> MGLNFFRKAAPEVRTEPVAERKASVTGRIVAMASGAGRPVWGPRDTVSLMRTGFAGNPVGFRSVKLIAEATAAVPLICQDAERRYEIHPVLDLLRRPNAGQGRAELFEALIGQILLSGNGYLEAVCPEPGVPRELHVLRSDRMAVVPGADGWPVGYDYTVGGRKHRFDMTGHPDPICHIKSFHPTDDHYGLSPMQAAAVALDVHNAASAWSKALLDNAARPSGAIIYKGADGQGVLAPEQYERLIFEMETHHQGARNAGRPMLLEGGLDWKPMGFSPSDMEFHETKAAAAREIALAFGVPPMLIGIPGDATYANYAEANRAFYRLTVLPLLTRVSAALAWWLSGYLGAQIELKPDLDQVPALAVERDQLWARIGAAGFLSNSEKRVLLGLPPT;> MMLNEVTAVPGTALPVAEFRDHLRLGTGFADLGAEDAALLSYLRAAIAAIEGRTAKALISRGFRLALTAWRWGDMQTLPIAPVATVTALRLVDAAGVETPVAAGWRLVPDMARPRIEALGAMLPMIPTGGRVEIDFTAGFGASWSALPVDLAQAVFLLAAQYYELRHDGAAEGGAMPFGVMALIERWRTVRVLGGRP

Gene transfer agents (GTAs) are DNA-containing phage-like particles produced by some species of bacteria and archaea. The genes encoding proteins that form Rhodobacter capsulatus GTA particles (RcGTA) are derived from phage DNA, which has been integrated into the bacterial genome. Here, we use cryo-electron microscopy (cryo-EM) to determine the structures of RcGTA before and after DNA ejection, and to visualize the interactions of RcGTA with R. capsulatus cells. Particles of RcGTA have heads with a diameter of 38-nm and 49-nm long tails.

The RcGTA head contains a special vertex in which a dodecamer of portal protein subunits (Rcc01684, g3) replaces a pentamer of major capsid proteins. The structure of the portal complex with imposed twelvefold symmetry was determined to a resolution of 3.3 Å. The portal complex is cone-shaped and contains a central channel with a diameter of 28 Å at its narrowest point. According to the convention established for the portal proteins of phages, the portal of RcGTA can be divided into the clip, stem, wing, and crown domains. A dodecamer of adaptor proteins (Rcc01688, g6) is attached to the surface of the portal complex exposed on the outside of the head and the adjacent part of the RcGTA capsid. The structure of the adaptor complex with imposed twelvefold symmetry was determined to a resolution of 3.3 Å. The maximum outer diameter of the adaptor complex is 143 Å and the minimum inner diameter is 35 Å. The adaptor protein can be divided into four domains: the attachment domain composed of β-strands 1–5, the tube domain formed by α-helices 1–4, the adaptor loop, and the C-terminal hook. Residues 175–197 from the C-terminal hook of the adaptor protein interact with helix α8 from the clip domain of the portal complex.>MDFYYMPGGGGCRTVIMVAKALGLELNKKLLNTMEGEQLKPEFVKLNPQHTIPTLVDNGFSIWESRAIAVYLVEKYGKDDYLLPNDPKKRAVINQRLYFDMGTLYESFAKYYYPLFRTGKPGSDEDLKRIETAFGFLDTFLEGQEYVAGDQLTV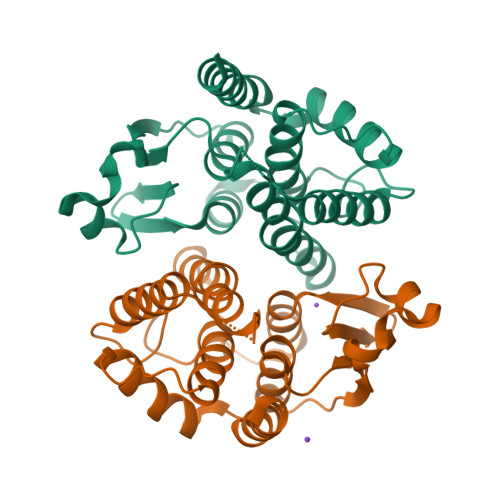ADIAILSTVSTFEVSEFDFSKYSNVSRWYDNAKKVTPGWDENWEGLMAMKALFDARKLAAK[2x]> VRWARALYDFEALEEDELGFRSGEVV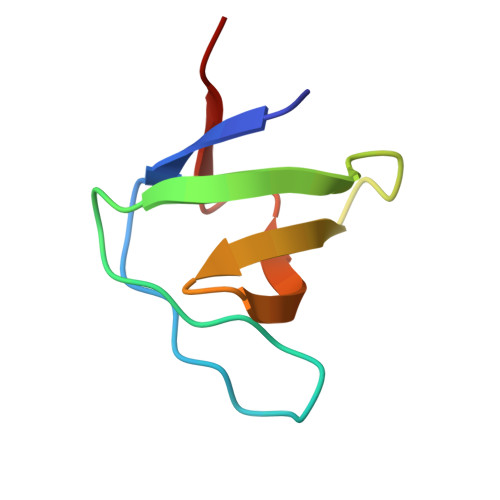EVLDSSNPSWWTGRLHNKLGLFPANYVAPMMR>QQVPILEKFCFTPHTEEGCLSERAALQEELQLCKGLVQALQTKVTQQGLKMVVPGLDGAQIPRDPSQQELPRLLSAACRLQLNGNLQLELAQVLAQERPKLPEDPLLSGLLDSPALKACLDTAVENMPSLKMKVVEVLAGHGHLYSRIPGLLSPHPLLQLSYTATDRHPQALEAAQAELQQHDVAQGQWDPADPAPSALGSADLLVCNCAVAALGDPASALSNMVAALREGGFLLLHTLLRGHPLGDIVAFLTSTEPQYGQGILSQDAWESLFSRVSLRLVGLKKSFYGSTLFLCRRPTPQDSPIFLPVDDTSFRWVESLKGILADEDSARPVWLKAINCATSGVVGLVNCLRREPGGNRLRCVLLSNLSSTSHVPEVDPGSAELQKVLQGDLVMNVYRDGAWGAFRHFLLEEDKGSKTFCPAHKSYIIAGGLGGFGLELAQWLIQRGVQKLVLTSRSGIRTGYQAKQVRRWRRQGVQVQVSTSNISSLEGARGLIAE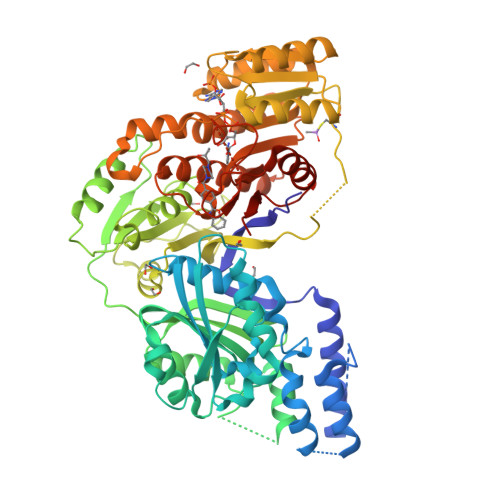AAQLGPVGGVFNLAVVLRDGLLENQTPEFFQDVCKPKYSGTLNLDRVTREACPELDYFVVFSSVSCGRGNAGQSNYGFANSAMERICEKRRHEGLPGLAVQWGAIGDVGILVETMSTNDTIVSGTLPQRMASCLEVLDLFLNQPHMVLSSFVLAEKHHHHHH[2x]> MAKILEGPAMKLFNKWGIPVPNYVVIMDPDRLAQLGEANKWLRESKLVVKAHEAIGGRFKLGLVKIGLNLEQAIEAAKEMLGAKVGTAEIGQVIIAEMLEHDAEFYVSIIGNKDGAELLISKHGGVDIEDNWDSVRRIQIELDENPTIEQLTELAKDAGFEGEIAERVGKICSRLILCFDNEDAQSIEINPLVIRKSDMRFAALDAVMNVDYDARFRHADWDFKPVSEIGRPFTEAEQQIMEIDSRIKGSVKFVEVPGGEIALLTAGGGASVFYADAVVARGGTIANYAEYSGDPADWAVEALTETICRLPNIKHIIVGGAIANFTDVKATFSGIINGFRESKSKGYLEGVKIWVRRGGPNEAQGLAAIKQLQEEGFDIHVYDRS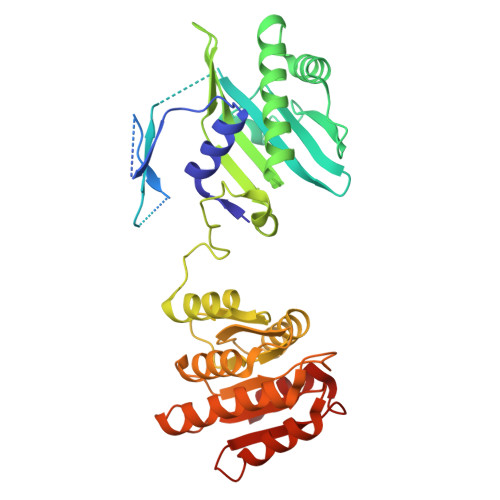MPMTDIVDLAMKS(3R)-3,5,5-trihydroxy-3-methylpentanoic acid 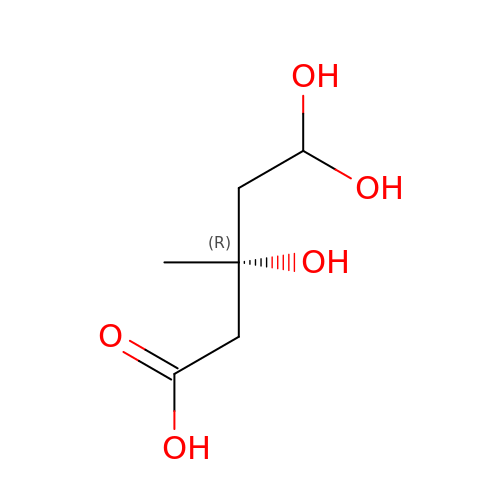| C6 H12 O5 | LENSSSSJMZWHIU-ZCFIWIBFSA-N>GGC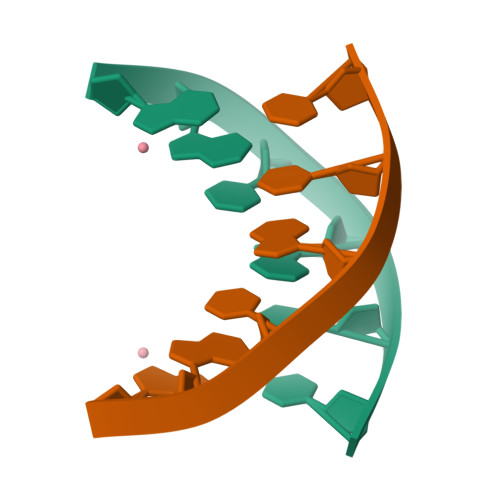GCC[5x]>[5x]GAMGMKQYIWLNETIKSNKQLAGPRGSYKRPVSVDIFRSSTILDPDKNYLLIVEEFHLHKIRLPLFKPAGHDYQVGIFNRSTDEIMGVREVDFSTFVDEDGYMYDYVDVGTAINETLAGLCDGIIGEEDIPVFSFNKHSKKFEITTTENFRNGHFIMFNDDM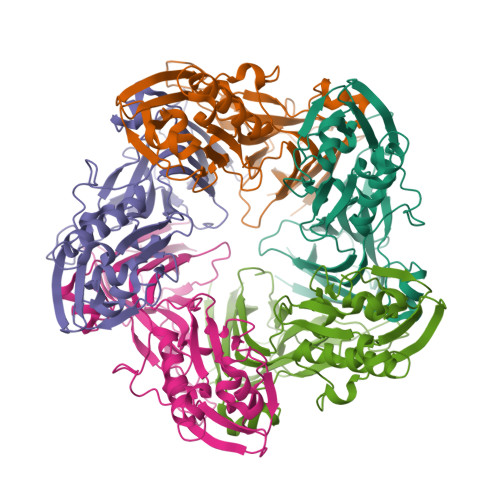RVDFNSFEFDDIDEEYSLVILNEDVETQDASTLEFLTPISHIVIESNDLPVSYELLPSISKNTTISDNTGVFLTNYKYLQQNNQDYNSILFRVENSSNKYHNILQTNFNRFNLSFTIYDYDNEKHPLTLLPQTVIQLKLLFESID>[4x]MYKVKVYVSLKESVLDPQGSAVQHALHSMTYNEVQDVRIGKYMEL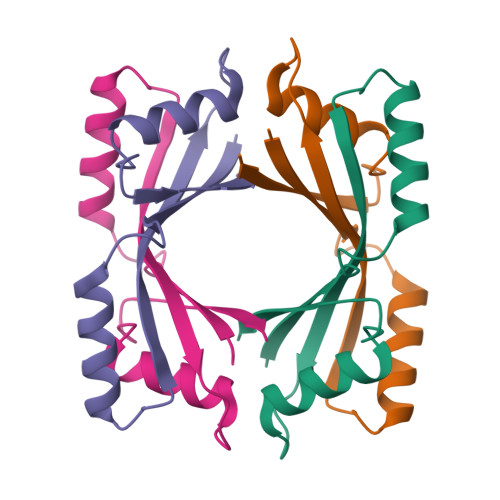TIEKSDRDLDVLVKEMCEKLLANTVIEDYRYEVEEVVAQ Two lysosomal proteins, NPC1 and NPC2, collaborate to export cholesterol from the lysosomal membrane. Human NPC1 has 1278 amino-acid residues, including an N-terminal lumenal domain (NTD), a middle lumenal domain (MLD), a C-terminal lumenal domain (CTD), and 13 TMs. Then, NPC1 employs its NTD and MLD to bind NPC2 and transfer its cholesterol.

To enhance the signal of itraconazole in the density map, we synthesized Br-labeled itraconazole (I-Br) which contains four cis-stereoisomers. The structure was then determined at 4.0-Å resolution from ~210 k particles. The isomers are indistinguishable at this resolution and they have similar interactions with the binding pocket; therefore, we built a model using the Br-labeled cis-2R,4 S,2′S isomer as a representative of the Br-labeled itraconazole mixture. The I-Br binds to a hydrophobic cavity that is generated by the SSD, the MLD and the CTD in the center of NPC1. Residues in the N-terminal loop and C-terminal helices of the MLD and the CTD, as well as TMs 3, 4, 5, and 13 contribute to the cavity that accommodates I-Br. The terminal sec-butyl moiety of I-Br inserts into the cavity and is contacted by residues W381, I609, L613, I685, F1087, I1220, and Y1225. Superimposing the cryo-EM structure of I-Br-bound NPC1 to the crystal structure of NPC1-ΔNTD reveals subtle differences between the TMs and no noticeable conformation changes between lumenal domains. Calculations using the program MOLE confirm a ~120-Å long tunnel in NPC1 with a minimum diameter of 7 Å, extending from the bottom of the MLD and CTD to the SSD. Our structural analysis reveals that P691 is located at the exit of the putative transport tunnel. Itraconazole may prevent this transport through blocking the tunnel directly.

> MTARGLALGLLLLLLCPAQVFSQSCVWYGECGIAYGDKRYNCEYSGPPKPLPKDGYDLVQELCPGFFFGNVSLCCDVRQLQTLKDNLQLPLQFLSRCPSCFYNLLNLFCELTCSPRQSQFLNVTATEDYVDPVTNQTKTNVKELQYYVGQSFANAMYNACRDVEAPSSNDKALGLLCGKDADACNATNWIEYMFNKDNGQAPFTITPVFSDFPVHGMEPMNNATKGCDESVDEVTAPCSCQDCSIVCGPKPQPPPPPAPWTILGLDAMYVIMWITYMAFLLVFFGAFFAVWCYRKRYFVSEYTPIDSNIAFSVNASDKGEASCCDPVSAAFEGCLRRLFTRWGSFCVRNPGCVIFFSLVFITACSSGLVFVRVTTNPVDLWSAPSSQARLEKEYFDQHFGPFFRTEQLIIRAPLTDKHIYQPYPSGADVPFGPPLDIQILHQVLDLQIAIENITASYDNETVTLQDICLAPLSPYNTNCTILSVLNYFQNSHSVLDHKKGDDFFVYADYHTHFLYCVRAPASLNDTSLLHDPCLGTFGGPVFPWLVLGGYDDQNYNNATALVITFPVNNYYNDTEKLQRAQAWEKEFINFVKNYKNPNLTISFTAERSIEDELNRESDSDVFTVVISYAIMFLYISLALGHMKSCRRLLVDSKVSLGIAGILIVLSSVACSLGVFSYIGLPLTLIVIEVIPFLVLAVGVDNIFILVQAYQRDERLQGETLDQQLGRVLGEVAPSMFLSSFSETVAFFLGALSVMPAVHTFSLFAGLAVFIDFLLQITCFVSLLGLDIKRQEKNRLDIFCCVRGAEDGTSVQASESCLFRFFKNSYSPLLLKDWMRPIVIAIFVGVLSFSIAVLNKVDIGLDQSLSMPDDSYMVDYFKSISQYLHAGPPVYFVLEEGHDYTSSKGQNMVCGGMGCNNDSLVQQIFNAAQLDNYTRIGFAPSSWIDDYFDWVKPQSSCCRVDNITDQFCNASVVDPACVRCRPLTPEGKQRPQGGDFMRFLPMFLSDNPNPKCGKGGHAAYSSAVNILLGHGTRVGATYFMTYHTVLQTSADFIDALKKARLIASNVTETMGINGSAYRVFPYSVFYVFYEQYLTIIDDTIFNLGVSLGAIFLVTMVLLGCELWSAVIMCATIAMVLVNMFGVMWLWGISLNAVSLVNLVMSCGISVEFCSHITRAFTVSMKGSRVERAEEALAHMGSSVFSGITLTKFGGIVVLAFAKSQIFQIFYFRMYLAMVLLGATHGLIFLPVLLSYIGPSVNKAKSCATEERYKGTERERLLNFWSHPQFEK The L-arginine biosynthesis pathway consists of eight enzymes that catalyse the conversion of L-glutamate to L-arginine, appears to be attractive target for anti-Tuberculosis (TB) drug discovery. The arginine biosynthesis pathway consists of eight different enzymes ([Fig fig1]) all considered to be essential for *M. tuberculosis* growth *in vitro*. In this work, the ligandability of four enzymes of the pathway ArgB, ArgC, ArgD and ArgF is explored using a fragment-based approach. In conclusion, using a fragment-based approach, we have discovered inhibitors that bind to novel sites in ArgB and ArgF and to the active sites of ArgC and ArgD, which in case of ArgB show on target activity against *M. tuberculosis*.

(A) X-ray crystal structure of ArgC apoenzyme superposed with the NAPD bound holoenzyme. Binding of NAPD causes significant structural changes in two loops of the protein that move from a closed to open conformation ([Fig fig2]). The apoenzyme ArgC with 5% DMSO was found to have a melting temperature of 67.7 °C. While 1 mM NADP^+^ gave a small average positive thermal shift of ~0.6 °C and 1 mM NADPH produced an average negative thermal shift of −0.9 °C across all DSF runs performed.

>ATKVAVAGASGYAGGEILRLLLGHPAYADGRLRIGALTAATSAGSTLGEHHPHLTPLAHRVVEPTEAAVLGGHDAVFLALPHGHSAVLAQQLSPETLIIDCGADFRLTDAAVWERFYGSSHAGSWPYGLPELPGARDQLRGTRRIAVPGCYPTAALLALFPALAADLIEPAVTVVAVSGTSGAGRAATTDLLGAEVIGSARAYNIAGVHRHTPEIAQGLRAVTDRDVSVSFTPVLIPASRGILATCTARTRSPLSQLRAAYEKAYHAEPFIYLMPEGQLPRTGAVIGSNAAHIAVAVDEDAQTFVAIAAIDNLVKGTAGAAVQSMNLALGWPETDGLSVVGVAP[4x]(2S,3S,4R,5S,2'S,3'S,4'R,5'S)-2,2'-(butane-1,4-diyl)bis(5-methylpyrrolidine-3,4-diol) 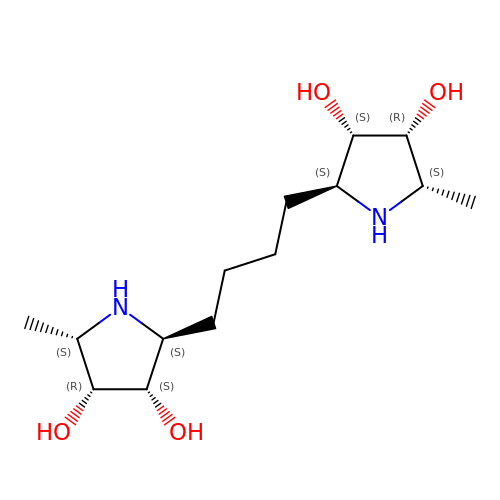| C14 H28 N2 O4 | FSZVPMVCORPBFY-OPEDVLRTSA-N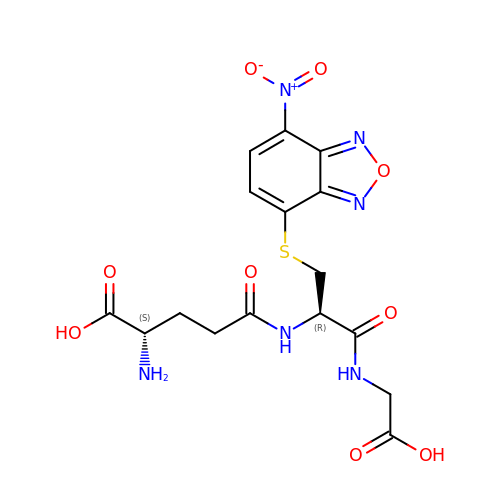(2~{S})-2-azanyl-5-[[(2~{R})-1-(2-hydroxy-2-oxoethylamino)-3-[(7-nitro-2,1,3-benzoxadiazol-4-yl)sulfanyl]-1-oxidanylidene-propan-2-yl]amino]-5-oxidanylidene-pentanoic acid | C16 H18 N6 O9 S | DLEOMDYTCAPLNH-YUMQZZPRSA-N>MAPVLSKDVADIESILALNPRTQSHAALHSTLA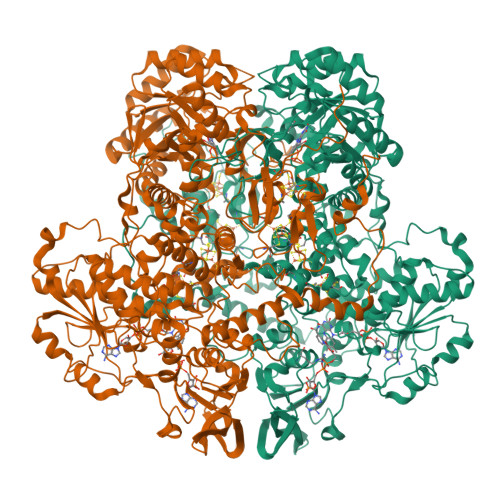KKLDKKHWKRNPDKNCFHCEKLENNFDDIKHTTLGERGALREAMRCLKCADAPCQKSCPTHLDIKSFITSISNKNYYGAAKMIFSDNPLGLTCGMVCPTSDLCVGGCNLYATEEGSINIGGLQQFASEVFKAMNIPQIRNPCLPSQEKMPEAYSAKIALLGAGPASISCASFLARLGYSDITIFEKQEYVGGLSTSEIPQFRLPYDVVNFEIELMKDLGVKIICGKSLSENEITLNTLKEEGYKAAFIGIGLPEPKTDDIFQGLTQDQGFYTSKDFLPLVAKSSKAGMCACHSPLPSIRGAVIVLGAGDTAFDCATSALRCGARRVFLVFRKGFVNIRAVPEEVELAKEEKCEFLPFLSPRKVIVKGGRIVAVQFVRTEQDETGKWNEDEDQIVHLKADVVISAFGSVLRDPKVKEALSPIKFNRWDLPEVDPETMQTSEPWVFAGGDIVGMANTTVESVNDGKQASWYIHKYIQAQYGASVSAKPELPLFYTPVDLVDISVEMAGLKFINPFGLASAAPTTSSSMIRRAFEAGWGFALTKTFSLDKDIVTNVSPRIVRGTTSGPMYGPGQSSFLNIELISEKTAAYWCQSVTELKADFPDNIVIASIMCSYNKNDWMELSRKAEASGADALELNLSSPHGMGERGMGLACGQDPELVRNICRWVRQAVQIPFFAKLTPNVTDIVSIARAAKEGGADGVTATNTVSGLMGLKADGTPWPAVGAGKRTTYGGVSGTAIRPIALRAVTTIARALPGFPILATGGIDSAESGLQFLHSGASVLQVCSAVQNQDFTVIQDYCTGLKALLYLKSIEELQGWDGQSPGTESHQKGKPVPRIAELMGKKLPNFGPYLEQRKKIIAEEKMRLKEQNAAFPPLERKPFIPKKPIPAIKDVIGKALQYLGTFGELSNIEQVVAVIDEEMCINCGKCYMTCNDSGYQAIQFDPETHLPTVTDTCTGCTLCLSVCPIIDCIRMVSRTTPYEPKRGLPLAVNPVC[4x]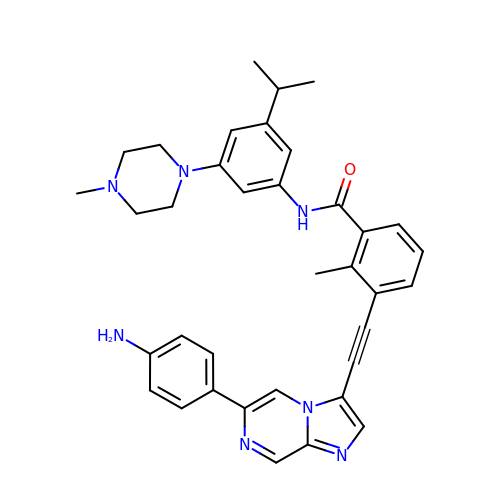3-[2-[6-(4-aminophenyl)imidazo[1,2-a]pyrazin-3-yl]ethynyl]-2-methyl-~{N}-[3-(4-methylpiperazin-1-yl)-5-propan-2-yl-phenyl]benzamide | C36 H37 N7 O | VBGZPGTYAGJBAX-UHFFFAOYSA-N> MFLYNLTLQRATGISFAIHGNFSGTKQQEIVVSRGKILELLRPDPNTGKVHTLLTVEVFGVIRSLMAFRLTGGTKDYIVVGSDSGRIVILEYQPSKNMFEKIHQETFGKSGCRRIVPGQFLAVDPKGRAVMISAIEKQKLVYILNRDAAARLTISSPLEAHKANTLVYHVVGVDVGFENPMFACLEMDYEEADNDPTGEAAANTQQTLTFYELDLGLNHVVRKYSEPLEEHGNFLITVPGGSDGPSGVLICSENYITYKNFGDQPDIRCPIP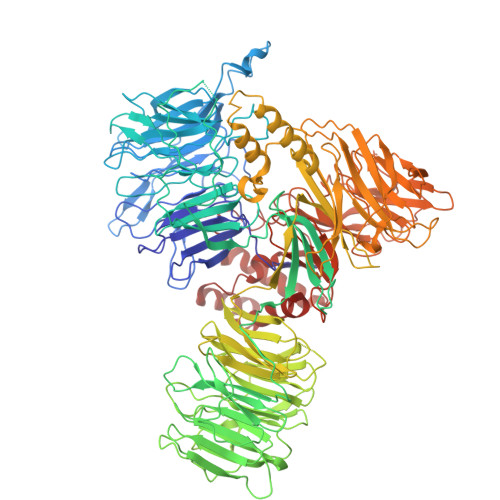RRRNDLDDPERGMIFVCSATHKTKSMFFFLAQTEQGDIFKITLETDEDMVTEIRLKYFDTVPVAAAMCVLKTGFLFVASEFGNHYLYQIAHLGDDDEEPEFSSAMPLEEGDTFFFQPRPLKNLVLVDELDSLSPILFCQIADLANEDTPQLYVACGRGPRSSLRVLRHGLEVSEMAVSELPGNPNAVWTVRRHIEDEFDAYIIVSFVNATLVLSIGETVEEVTDSGFLGTTPTLSCSLLGDDALVQVYPDGIRHIRADKRVNEWKTPGKKTIVKCAVNQRQVVIALTGGELVYFEMDPSGQLNEYTERKEMSADVVCMSLANVPPGEQRSRFLAVGLVDNTVRIISLDPSDCLQPLSMQALPAQPESLCIVEMGGTEKQDELGERGSIGFLYLNIGLQNGVLLRTVLDPVTGDLSDTRTRYLGSRPVKLFRVRMQGQEAVLAMSSRSWLSYSYQSRFHLTPLSYETLEFASGFASEQCPEGIVAISTNTLRILALEKLGAVFNQVAFPLQYTPRKFVIHPESNNLIIIETDHNAYTEATKAQRKQQMAEEMVEAAGEDERELAAEMAAAFLNENLPESIFGAPKAGNGQWASVIRVMNPIQGNTLDLVQLEQNEAAFSVAVCRFSNTGEDWYVLVGVAKDLILNPRSVAGGFVYTYKLVNNGEKLEFLHKTPVEEVPAAIAPFQGRVLIGVGKLLRVYDLGKKKLLRKCENKHIANYISGIQTIGHRVIVSDVQESFIWVRYKRNENQLIIFADDTYPRWVTTASLLDYDTVAGADKFGNICVVRLPPNTNDEVDEDPTGNKALWDRGLLNGASQKAEVIMNYHVGETVLSLQKTTLIPGGSESLVYTTLSGGIGILVPFTSHEDHDFFQHVEMHLRSEHPPLCGRDHLSFRSYYFPVKNVIDGDLCEQFNSMEPNKQKNVSEELDRTPPEVSKKLEDIRTRYAF> MSLRPSAKTEVRRNRYKVAVDAEEGRRRREDNLVEIRKNKREENLQKKRFTSSMAFGSATGQTEQDLSSANQLKDNLPAMVAGIWSEDSNSQLEATNLLRKLLSIEQNPPINEVVQSGVVPRVVKFLSRDDFPKLQFEAAWALTNIASGTSENTNVIIESGAVPIFIQLLSSASEDVREQAVWALGNVAGDSPKCRDLVLSYGAMTPLLSQFNENTKLSMLRNATWTLSNFCRGKPPPAFEQTQPALPVLERLVQSMDEEVLTDACWALSYLSDNSNDKIQAVIEAGVVPRLIQLL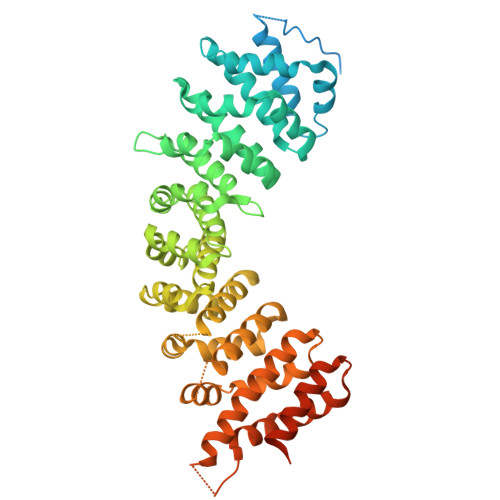GHSSPSVLIPALRTIGNIVTGDDLQTQMVLDQQALPCLLNLLKNNYKKSIKKEACWTISNITAGNADQIQAVIDAGIIQSLVWVLQSAEFEVKKEAAWGISNATSGGTHDQIKFMVSQGCIKPLCDLLTCPDLKVVTVCLEALENILVVGEAEKNLGHTGEDNLYAQMIDEAEGLEKIENLQSHDNNDIYDKAVKILETFWTEDNEEEGNDENHAPQSGFQFGSTNVPPGQFNFI> NPVENYIDEVLNEVLVVPNINSSNPTTSNSAPALDAAETGHTSSVQPEDVIETRYVQTSQTRDEMSLESFLGRSGCIHESKLEVTLANYNKENFTVWAINLQEMAQIRRKFELFTYTRFDSEITLVPCISALSQDIGHITMQYMYVPPGAPVPNSRDDYAWQSGTNASVFWQHGQAYPRFSLPFLSVASAYYMFYDGYDEQDQNYGTANTNNMGSLCSRIVTEKHIHKVHIMTRIYHKAKHVKAWCPRPPRALEYTRAHRTNFKIEDRSIQTAIVTRPIITTA;> SPTVEACGYSDRIIQITRGDSTITSQDVANAIVAYGVWPHYLSSKDASAIDKPSQPDTSSNRFYTLRSVTWSSSSKGWWWKLPDALKDMGIFGENMFYHYLGRSGYTIHVQCNASKFHQGTLIVALIPEHQIASALHGNVNVGYNYTHPGETGREVKAETRLNPDLQPTEEYWLNFDGTLLGNITIFPHQFINLRSNNSATIIAPYVNAVPMDSMRSHNNWSLVIIPICPLETSSAINTIPITISISPMCAEFSGARAKRQ;> GLPVFITPGSGQFLTTDDFQSPCALPWYHPTKEISIPGEVKNLVEICQVDSLVPINNTDTY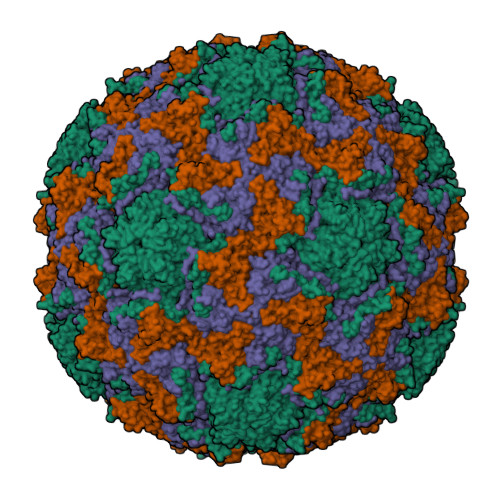INSENMYSVVLQSSINAPDKIFSIRTDVASQPLATTLIGEISSYFTHWTGSLRFSFMFCGTANTTVKLLLAYTPPGIAEPTTRKDAMLGTHVIWDVGLQSTISMVVPWISASHYRNTSPGRSTSGYITCWYQTRLVIPPQTPPTARLLCFVSGCKDFCLRMARDTNLHLQSGAIAQ;> MGAQVSRQNVGTHSTQNSVSNGSSLNYFNINYFKDAASNGASKLEFTQDPSKFTDPVKDVLEKGIPTLQ>VSRIVVHTRWASNVDFDRDSSVIMAPPTENNIHLFKQLLNTETLSVRGANPLMFRANVLHMLLEFVLDNLYLNRHTGFSQDHTPFTEGANLRSLPGPDAEKWYSIMYPTRMGTPNVSKICNFVASCVRNRVGRFDRAQMMNGAMSEWVDVFETSDALTVSIRGRWMARLARMNINPTEIEWALTECAQGYVTVTSPYAPSVNRLMPYRISNAERQISQIIRIMNIGNNATVIQPVLQDISVLLQRISPLQIDPTIISNTMSTVSESTTQTLSPASSILGKLRPSNSDFSSFRVALAGWLYNGVVTTVIDDSSYPKDGGSVTSLENLWDFFILALALPMTTDPCAPVKAFMTLANMMVGFETIPMDNQIYTQSRRASAFSTPHTWPRCFMNIQLISPIDAPILRQWAEIIHRYWPNPSQIRYGAPNVFGSANLFTPPEVLLLPIDHQPANVTTPTLDFTNELTNWRARVCELMKNLVDNQRYQPGWTQSLVSSMRGTLDKLKLIKSMTPMYLQQLAPVELAVIAPMLPFPPFQVPYVRLDRDRVPTMVGVTRQSRDAITQPALSLSTTNTTVGVPLALDARAITVALLSGKYPPDLVTNVWYADAIYPMYADTEVFSNLQRDMITCEAVQTLVTLVAQISDTQYPVDRYLDWIPSLRASAATAATFAEWVNTSLKTAFDLSDMLLEPLLSGDPRMTQLAIQYQQYNGRTFDVIPEMPGSVIADCVQLTAEVFNHEYNLFGIARGDIIIGRVQSTHLWSPLAPPPDLVFDRDTPGVHIFGRDCRISFGMNGAAPMIRDETGMMVPFEGNWIFPLALWQMNTRYFNQQFDAWIKTGELRIRIEMGAYPYMLHYYDPRQYANAWNLASAWLEEITPTSIPSVPFMVPISSDHDISSAPAVQYIISTEYNDRSLFCTNSSSPQTIAGPDKHIPVERYNILTNPDAPPTQIQLPEVIDLYNVVTRYAYETPPITAVVMGVP[2x]

The particles harbour 10-separate genome segments and comprise two principle protein layers, the innermost composed of 120 copies of protein λ1 clamped together by 150 copies of σ2 (viral polymerases, λ3, are attached inside adjacent to the icosahedral fivefold axes). The outer layer consists of 600 copies each of μ1 and σ3. The array of μ1 and σ3 is interrupted at the fivefold axes by pentameric λ2 turrets which enzymatically cap the mRNA transcripts produced by the polymerase on egress from the particle. Here we demonstrate that vitrification of infected cells followed by cryo-focussed ion beam (cryo-FIB) milling and cryo-electron tomography (cryo-ET) allows high resolution reconstruction of assembly intermediates of a mammalian reovirus, allowing atomic models to be constructed which throw light on some of these fundamental questions.

Unexpectedly, numerous star shaped particles were observed in the virus factories in addition to particles consistent with the expected virion architecture. For stars, analysis focused on the fivefold regions using emClarity16 yielded a reconstruction at 6.6 Å. Broad features of the organisation of the molecules parallel the arrangement seen in the virus—five copies of λ1 (termed A molecules) cluster around each fivefold axis and five further copies of λ1 (termed B), orientated in a similar fashion to the A molecules, are located 35 Å further from the fivefold. Since the 60 copies each of the A and B molecules account for the large majority of the density for these particles we henceforth term them single-layered particles (SLPs). The maximum diameter of the SLPs is very similar to the corresponding layer of virion-like particles, however whilst the latter are roughly spherical the SLP is collapsed inwards at the icosahedral fivefolds by 100 Å, to give the characteristic star shaped cross-section. Superposition of equivalent λ1 molecules between the virion-like particles and SLPs shows that the majority of the movement is caused by molecules A and B tipping inwards by ~35°. There are also significant conformational changes within the molecules, the largest being a hinge-like flexing of two parts of the subunit (the same hinge is used to adjust between the A and B conformations in the virus particles). The molecules rotate by some 35° and slide partially over each other like the blades of a camera iris. Overall the λ1 protein structure allows it to occupy two radically different configurations in the SLP/virion-like particle, but is likely not compatible with stable intermediate structures. The interior volume of the SLP is 59% of that of the virion-like particle, thus the dsRNA genome segments cannot fit inside (the dsRNA in the core of the Reoviridae is already at a concentration of ~410 mg/ml5).4-chloro-N-[(3S,4R)-4-phenylpyrrolidin-3-yl]-3-{[(1H-pyrrolo[2,3-b]pyridin-5-yl)oxy]methyl}benzamide 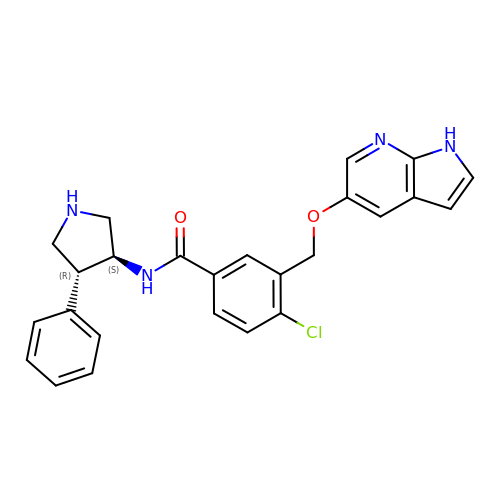| C25 H23 Cl N4 O2 | XQBVNNMIIVBLPN-JTHBVZDNSA-N In most bacterial species, faithful chromosome segregation is mediated by the tripartite ParA-ParB-parS system. ParB, a CTPase and DNA-binding protein, nucleates on parS before spreading to adjacent non-specific DNA to form a higher-order nucleoprotein complex. The ParB-DNA nucleoprotein complex stimulates the ATPase activity of ParA, driving the movement of the parS locus (and subsequently, the whole chromosome) to the opposite pole of the cell. ParB spreads by sliding along the DNA, in a manner that depends on the binding of a co-factor, cytidine triphosphate (CTP) (Balaguer F de et al., 2021; Jalal et al., 2020c; Osorio-Valeriano et al., 2019; Soh et al., 2019).

After screening several constructs with different lengths of ParB and parS, we obtained crystals of a 50 amino acid C-terminally truncated ParB in complex with a 22 bp parS DNA. This protein variant lacks the C-terminal domain (CTD) responsible for ParB dimerization (Figge et al., 2003). Diffraction data for the ParB∆CTD-parS co-crystal were collected to 2.9 Å resolution, and the structure was solved by molecular replacement. The asymmetric unit contains four copies of ParB∆CTD and two copies of the parS DNA. Each ParB∆CTD binds to a half parS site, but there is no protein-protein contact between the two adjacent subunits. We observed that helices α3 and α4 are packed towards the DBD and are connected to the rest of the NTD via an α3–β4 loop. While the DBD and helices α3–α4 are near identical between the two ParB∆CTD subunits (root-mean-square deviation [RMSD] = 0.19 Å, Figure 1C), the rest of the NTD, from α1 to β4, adopts notably different conformations in the two subunits. Specifically, NTDs (α1–β4) from the two ParB∆CTD subunits are related by a rotation of approximately 80o due to changes in a flexible loop in between α3 and β4. In the nucleating state, as represented by the ParB∆CTD-parS structure, helices α3 and α4 from each subunit bundle together (32o angle between α3 and α4). Nucleating ParB is an open clamp in which parS DNA is held tightly (nM affinity) at the DBD. The NTDs of nucleating ParB can adopt multiple alternative conformations, and crucially there is no contact between opposing NTDs.

>MSEGRRGLGRGLSALLGEVDAAPAQAPGEQLGGSREAPIEILQRNPDQPRRTFREEDLEDLSNSIREKGVLQPILVRPSPDTAGEYQIVAGERRWRAAQRAGLKTVPIMVRELDDLAVLEIGIIENVQRADLNVLEEALSYKVLMEKFERTQENIAQTIGKSRSHVANTMRLLALPDEVQSYLVSGELTAGHARAIAAAADPVALAKQIIEGGLSVRETEALARKAPNLSAGKSKGGRPPRVKDKLAAALEHHHHHH[4x]>[2x]MKTPEDCTGLA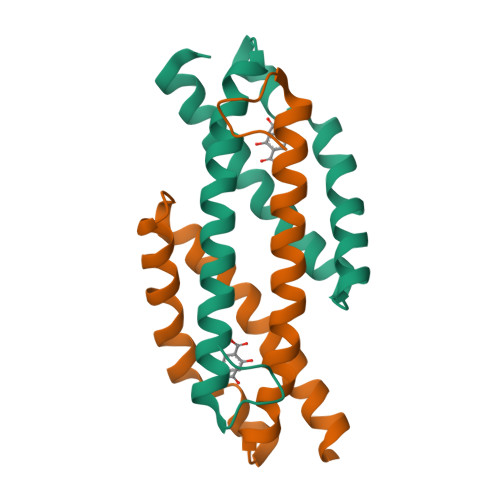DIREAIDRIDLDIVQALGRRMDYVKAASRFAASEAAIPAPERVAAMLPERARWAEENGLDAPFVEGLFAQIIHWYIAEQIKYWRQTRGAA>MRILVIEDEISLNKTIIDNLNEFGYQTDSSENFKDGEYFIGIRHYDLVLASWNLPDGDGAELVNTIKHKSPRTSVMIMSAKADKDTEIKALKAGADDFVKKPLDFDILLARIEARLRLGGTNVIKIEDLVIDPDEEKITYKGQDIELKGKPFEVLT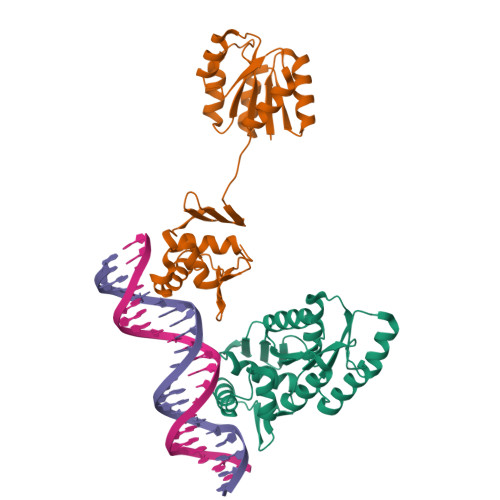HLARHSDQIVSKEQLLDAIWEEPELVTPNVIEVAINQIRQKMDKPLNISTIETVRRRGYRFCFPKKS[2x]>[4x]SMKALDELVFDNRFARLGDAFSTHVLPEPIDAPRLVVASESALALLDLAPEQSELPLFAEIFSGHKLWAEAEPRAMVYSGHQFGSYNPRLGDGRGLLLGEVYNDAGEHWDLHLKGAGRTPYSRMGDGRAVLRSSIREFLASEALHALGIPSSRAACVVSSNTPVWREKQE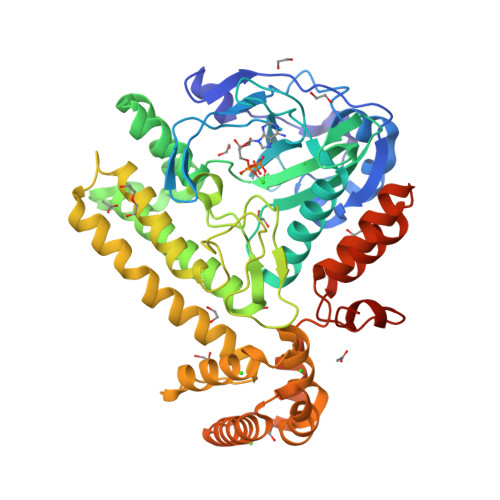YAAMVLRLAQSHVRFGSLEYLFYTKQPEHLKTLAEHVLTMHYPHCQEQPEPYLAMFREIVERNAELIAKWQAYGFCHGVMNTDNMSILGITFDFGPFAFLDDFDEHFICNHSDHEGRYSFSNQVPIAQWNLSALGQALTPFVSVEALRETIGLFLPLYQAHYLDLMRRRLGLTVAQDQDDKLVSQLLQLMQNSGVDYTLFFRRLGDQPAAQALRALRDDFVDIKVFDDWAQAYQARIAAEENGTEQARKERMHAVNPLYILRNYLAQNAIEAAEKGDYEEVRRLHQVLCTPFTEQPGMEGYAQRPPDWGKHLEISCSS> PQYQTWEEFSRAAEKLYLADPMKARVVLKYRHSDGNLCVKVTDDLVCLVYKTDQAQDVKKIEKF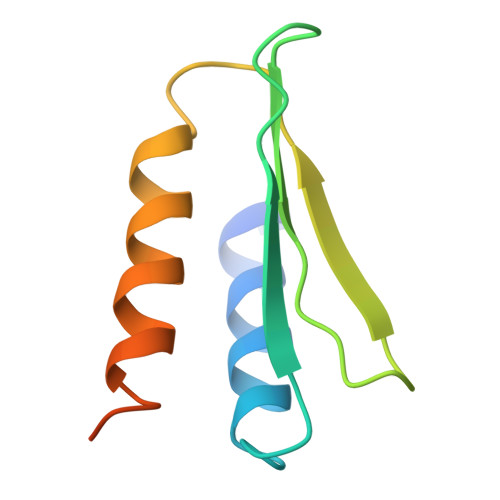HSQLMRLMVAKEARNVTMETE>[2x]LSTWQTFRRLWPTIAPFKAGLIVAGIALILNAASDTFMLSLLKPLLDDGFGKTDRSVLLWMPLVVIGLMI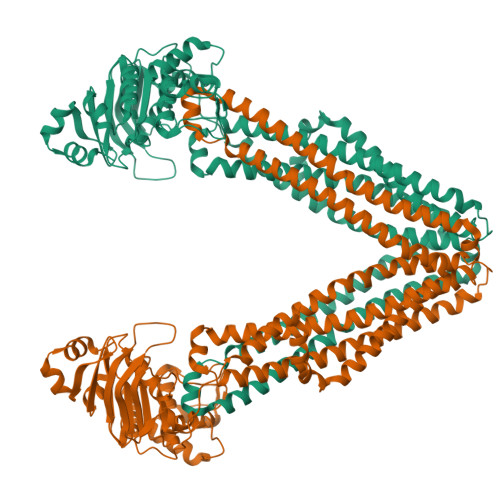LRGITSYISSYCISWVSGKVVMTMRRRLFGHMMGMPVAFFDKQSTGTLLSRITYDSEQVASSSSGALITVVREGASIIGLFIMMFYYSWQLSIILVVLAPIVSIAIRVVSKRFRSISKNMQNTMGQVTTSAEQMLKGHKEVLIFGGQEVETKRFDKVSNKMRLQGMKMVSASSISDPIIQLIASLALAFVLYAASFPSVMDSLTAGTITVVFSSMIALMRPLKSLTNVNAQFQRGMAACQTLFAILDSEQEKDEGKRVIDRATGDLEFRNVTFTYPGREVPALRNINLKIPAGKTVALVGRSGSGKSTIASLITRFYDIDEGHILMDGHDLREYTLASLRNQVALVSQNVHLFNDTVANNIAYARTEEYSREQIEEAARMAYAMDFINKMDNGLDTIIGENGVLLSGGQRQRIAIARALLRDSPILILDEATSALDTESERAIQAALDELQKNRTSLVIAHRLSTIEQADEIVVVEDGIIVERGTHSELLAQHGVYAQLHKMQFGQ The exo-β-1,3-galactanase is a glycoside hydrolase from the basidiomycete Phanerochaete chrysosporium (Pc1,3Gal43A), which specifically cleaves AGPs. In this context, exo-β-1,3-galactanase (EC 3.2.1.145) specifically cleaves the nonreducing end β-1,3–linked galactosyl linkage of β-1,3-galactans to release d-galactose (Gal). In this study, we solved the apo and liganded structures of Pc1,3Gal43A, which reveal a glycoside hydrolase family 43 subfamily 24 (GH43_sub24) catalytic domain together with a carbohydrate-binding module family 35 (CBM35) binding domain. The N-terminal catalytic domain consists of a five-bladed β-propeller (Gln21–Gly325), as in other GH clan-F enzymes, and the C-terminal domain (PcCBM35) takes a β-jellyroll fold (Thr326–Tyr448) structure, as in previously reported CBM35s.

The crystal structure of the SeMet derivative of Pc1,3Gal43A was first determined by means of the multiwavelength anomalous dispersion method, and this was followed by structure determination of the ligand-free WT, the WT bound with Gal (WT_Gal), the E208Q mutant co-crystallized with β-1,3-galactotriose (Gal3; E208Q_Gal3), and the E208A mutant co-crystallized with Gal3 (E208A_Gal3). In the catalytic site, the vibration levels of some residues were significantly different between the apo and holo forms. Tyr126, Arg157, Asp158, Asn179, Asn180, Gln181, Trp229, and Gln263 in the liganded structures showed smaller vibrations than in the apo structures. These results indicate that side-chain fluctuations converge upon ligand binding. The catalytic acid, Glu208, has two major conformations in WT and WT_Gal. These two conformations were also reported in the BT3683 structure. Thus, the movement of this residue appears to be important for catalysis. Based on the results of ensemble refinement, Trp229 showed huge fluctuation, especially in the apo structure. Asp158 of WT and E208A_Gal3 show greater vibration than WT_Gal and E208Q_Gal3. The role of Asp158 is thought to be a pKa modulator; therefore, its function and conformational stability might be related.

>[2x]NQIVSGAAWTDTAGNTIQAHGAGILQVGSTFYWFGEDKSHNSALFKAVSCYTSSDLVNWSRQNDALSPIAGTMISTSNVVERPKVIFNQKNSEYVMWFHSDSSNYGAAMVGVATAKTPCGPYTYKGSFKPLGADSRDESIFQDDDSAQTAYLLYASDNNQNFKISRLDANYYNVTAQVSVMNGATLEAPGIVKHNGEYFLIASHTSGWAPNPNKWFSASSLAGPWSAQQDIAPSATRTWYSQNAFDLPLGSNAIYMGDRWRPSLLGSSRYIWYPLDFSSGAPQIVHADVWSVNVQAGTYSVASGTSYEAENGQRGGSSTILSGSGFSGGKAVGYLGHGGTVTINNVQSNGGSHWVALYFANGDSTYRNVTVSVNGGPSVLVDQPDSGGGNVVISVPVKLNLNSGENSITFGSGQSNYAADLDKIIVY> MNERKKSI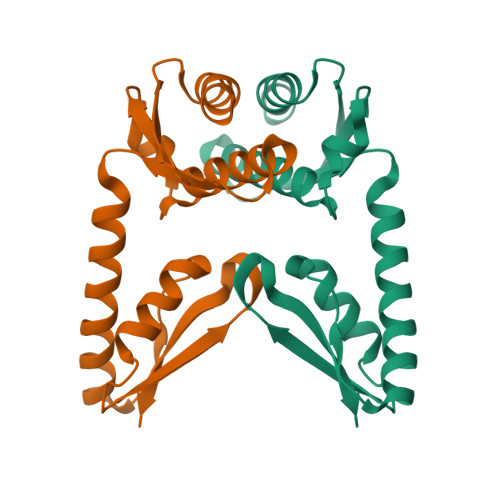DELLSDLGVLEEAPVEVELKESGTPEAQGDPRAFLEEFLGGLLLLLDPGHRLEVRVEGETLKAEVKGGDLGRFIGKEGRTLRAVEHLARVVLARRFGTGYRLVLDAAGYRSRAEARIRRLAEEAALTVAMTGEPLHLPPMPPGERRIVHMLLKNHPRVTTESQGEGEERHVVVYPRREAQG> DGDQCETSPCQNQGKCKDGLGEYT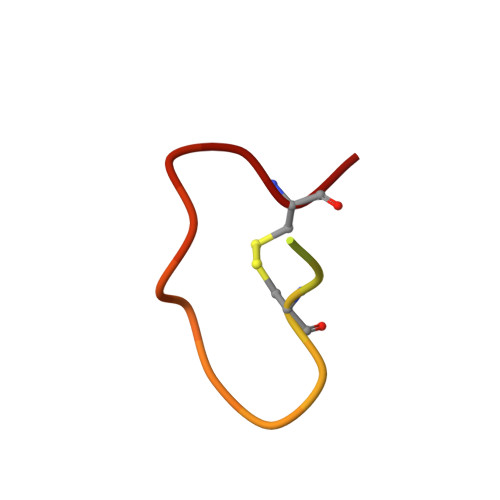CT>MGHHHHHHVSSTNGFSATRSTVIQLLNNISTKREVEQYLKYFTSVSQQQFAVIKVGGAIISDNLHELASCLAFLYHVGLYPIVLHGTGPQVNGRLEAQGIEPDYIDGIRITDEHTMAVVRKCFLEQNLKLVTALEQLGVRARPITSGVFTADYLDKDKYKLVGNIKSVTKEPIEASIKAGALPILTSLAETASGQMLNVNADVAAGELARVFEPLKIVYLNEKGGIINGSTGEKISMINLDEEYDDLMKQSWVKYGTKLKIREIKELLDYLPRSSSVAIINVQDLQKELFTDSGAGTMIRRGYKLVKRSSIGEFPSADALRKALQRDAGISSGKESVASYLRYLENSDFVSYADEPLEAVAIVK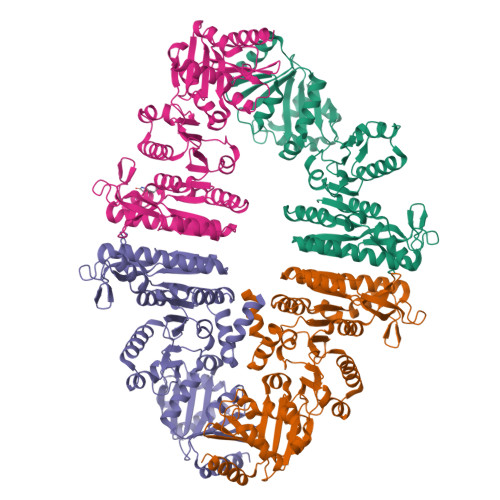KDTNVPTLDKFVCSDAAWLNNVTDNVFNVLRRDFPALQWVVSENDANIAWHFDKSQGSYLKGGKVLFWYGIDDINTISELVENFVKSCDTASTLNSSASS[8x]>GHMSGRGKKPTRTLVMTSMPSEKQNVVIQVVDKLKGFSIAPDVCETTTHVLSGKPLRTLNVLLGIARGCWVLSYDWVLWSLELGHWISEEPFELSHHFPAAPLCRSECHLSAGPYRGTLFADQPVMFVSPASSPPVAKLCELVHLCGGRVSQVPRQ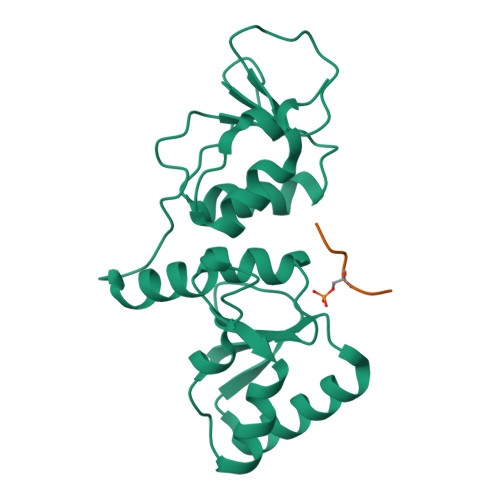ASIVIGPYSGKKKATVKYLSEKWVLDSITQHKVCAPENYLLSQ[8x];>[8x]KKATQASQEY> MSDGTSQPDGGNAVHSAARVERAADGPGGSGGGGSGGGGVGVSTGSYDNQTHYRFLGDGWVEITALATRLVHLNMPKSENYCRIRVHNTTDTSVKGNMAKDDAHEQIWTPWSLVDANAWGVWLQPSDWQYICNTMSQLNLVSLDQEIFNVVLKTVTEQDSGGQAIKIYNNDWTACMMVAVDSNNILPYTPAANSMETLGFYPWKPTIASPYRYYFCVDRDLSVTYENQEGTIEHNVMGTPKGMNSQFFTIENTQQITLLRTGDEFATGTYYFDTNPVKLTHTWQTNRQLGQPPLLSTFPEADTDAGTLTAQGSRHGATQMEVNWVSEAIRTRPAQVGFCQPHNDFEASRAGPFAAPKVPADVTQGMDREANGSVRYSYGKQHG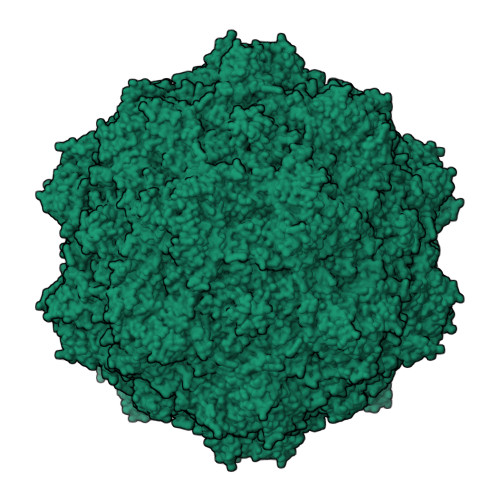ENWAAHGPAPERYTWDETNFGSGRDTRDGFIQSAPLVVPPPLNGILTNANPIGTKNDIHFSNVFNSYGPLTTFSHPSPVYPQGQIWDKELDLEHKPRLHITAPFVCKNNAPGQMLVRLGPNLTDQYDPNGATLSRIVTYGTFFWKGKLTMRAKLRANTTWNPVYQVSVEDNGNSYMSVTKWLPTATGNMQSVPLITRPVARNTY>[2x]GSHMITYKKLLDEL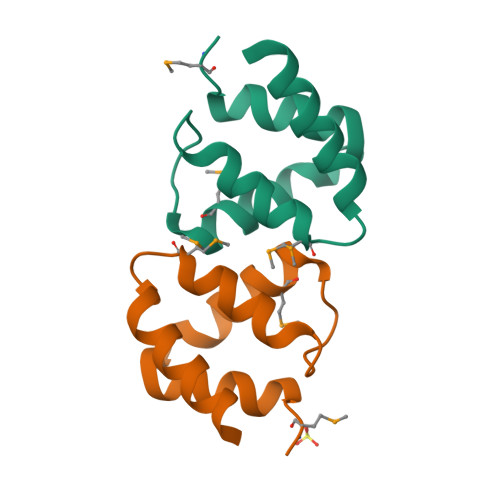KKEIGPIAKIFLNKAMESLGYDDVDDSNYKEILSVLKMNKELREYVEIVEERLEKEG>MTTTSPLHFVTLLGSLRKASFNAAVARALPEIAPEGIAITPLGSIGTFPHYSQDVQEEGFPAPVLTMAQQIATADAVVIVTPEYNYSVPGVLKNAIDWLSAVSPQPLAGKPVALVTASPGMIGGARAQYHLRQSLVFLDA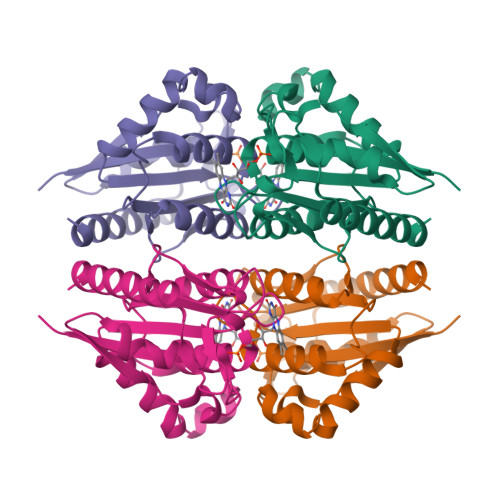YVLNRPEAMIGQVTGKVDAQTLELSDVATREFLARQLDALAALARTLSPRAITHHHHHH[12x]> GSARDISSTNVTDLTVSPSKIEDGGKTTVKMTFDDKNGKIQNGDMIKVAWPTSGTVKIEGYSKTVPLTVKGEQVGQAVITPDGATITFNDKVEKLSDVSGFAEFEVQGRNLTQTNTSDDKVATITSGNKSTNVTVHKSEAGTSSVFYYKTGDMLPEDTTHVRWFLNINNEKSYVSKDITIKDQIQGGQQLDLS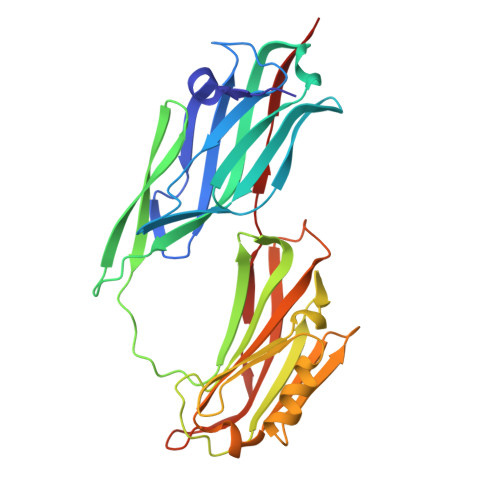TLNINVTGTHSNYYSGQSAITDFEKAFPGSKITVDNTKNTIDVTIPQGYGSYNSFSINYKTKITNEQQKEFVNNSQAWYQEHGKEEVNGKSFNHTVHNINANAGIEGTVK> AMAMNDLTLHYLYDPLCGWCYGASPLLAAACEVTGLDVRLHGGGMMTDANRQPVGAGLRHYVMPHDLRIAQLTGQPFGKDYFDGLLRDTSAVFDSAPPTAAVLAAEALDGLGAAMLARIQRAHYV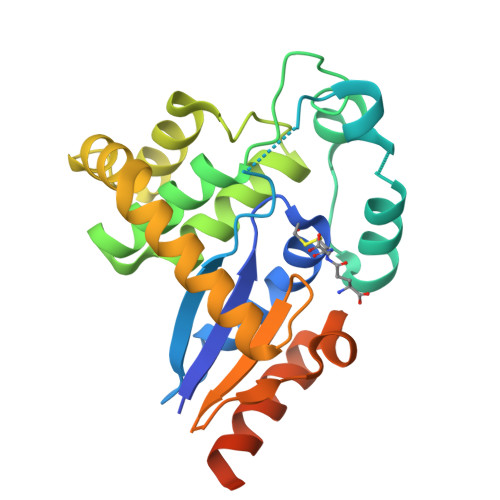EGRRIAERPVLLELGAELGLGEGFAEAFDACSGEPLRAHFADSRRLMNRLGAAGFPTFALERDGRLQVLDTGRYLGQPDDWRAFLETQLRLAGGSGAVGGAAAPLCRIDGCA> GDVVEAIEGAVARVADTISSGPTNSQAVPALTAVETGHTSQVVPGDTMQTRHVKNYHSRSESTIENFLSRSACVYMGEYYTTNTDETKRFASWTINARRMVQMRRKLEMFTYVRFDVEVTFVITSKQDQGTQLGQDMPPLTHQIMYIPPGGPIPKSTTDYAWQTSTNPSIFWTEGNAPPRMSIPFVSIGNAYSNFYDGWSHFSQNGVYGYNTLNNMGQLYMRHVNGPSPLPMTSIVRVYFKPKHVKAWVPRPPRLCQYKNASTVNFSSTNITDKRDSITHVPDTVKPDVTTH;> SPSAEECGYSDRVRSITLGNSTITTQECANVVVAYGRWPEYLSDKEATAEDQPTQPDVATCRFYTLESVTWEKDSPGWWWKFPDALKDMGLFGQNMYYHYLGRAGYTIHVQCNASKFHQGCLLVVCVPEAEMGCSDVGGTVNEHAISEGEIAKKFSATATNGAHTVQSIVTNAGMGVGVGNLTIYPHQWVNLRTNNSATIVMPYINSVPMDNMFRHHNFTLMIIPFVSLDYSSDASTYVPITVTVAPMCAEYNGLRLATSLQ;> GLPVMNTPGSNQFLTSDDFQSPSAMPQFDVTPELDIPGEVKNLMEIAEVDSVVPVNNVVGKLDTMDIFRIPVQSGNHQSTQVFGFQVQPGLDSVFKHTLLGEILNYYAHWSGSVKLTFVFCGSAMATGKFLLAYSPPGANAPKTRKDAMLGTHVIWDVGLQSSCVLCIPWISQTHYRLVHQDEYTSAGNVTCWYQTGIVVPAGTPTLCSIMCFVSACNDFSVRLLKDTPFIEQSALLQ;> MGAQVSTQKTGAHETGLNASGNSIIHYTNINYYKDAASNSANRQDFTQDPGKFTEPVKDIMIKSMPALN;> MGCVAETGDCGLPPDVPNAQPALEGRTSFPEDTVITYKCEESFVKIPGEKDSVICLKGSQWSDIEEFCNRSCEVPTRLNSASLKQPYITQNYFPVGTVVEYECRPGYRREPSLSPKLTCLQNLKWSTAVEFCKKKSCPNPGEIRNGQIDVPGGILFGATISFSCNTGYKLFGSTSSFCLISGSSVQWSDPLPECREIYCPAPPQIDNGIIQGERDHYGYRQSVTYACNKGFTMIGEHSIYCTVNNDEGEWSGPPPECRGGTKHHHHHH

Echoviruses, for which there are currently no approved vaccines or drugs, are responsible for a range of human diseases, for example echovirus 11 (E11) is a major cause of serious neonatal morbidity and mortality. Decay-accelerating factor (DAF, also known as CD55) is an attachment receptor for E11. The capsid consists of 60 identical protomers arranged with icosahedral symmetry and each protomer is composed of four capsid proteins, VP1–4, derived from the P1 polyprotein. DAF is one of the regulators of the complement system, inhibiting formation of the complement convertases in both the classical and alternative pathways.

The cryo-EM structure of the E11-DAF complex at neutral pH (pH 7.4) was determined at a nominal gold-standard resolution of 3.1 Å. In contrast the density for the DAF was weak. Whilst at low resolution the molecular envelope was clear, at high resolution the density became fragmentary at a contour level where the capsid density was still continuous. It was clear that this was in substantial part because the DAF bound close to the icosahedral 2-fold axes, so that at most only 30 DAFs could be bound per particle, in particular, SCR domains 2 and 3 of the 2-fold related DAF molecules clash. As expected for engagement with an attachment receptor with relatively weak binding (reported KD for E11 ∼3.0 μm), which is not responsible for internalisation and genome release, the E11 structure is in its un-expanded state with the natural pocket factor (modelled as sphingosine) bound in the VP1 pocket. DAF binds E11 at the southern rim of the canyon, rather than into the canyon itself. The footprint of the DAF receptor on the virus is ~900 Å2. The VP2 EF loop of E11 and SCR 3 of DAF dominate the interaction, although the VP3 BC loop of E11 and DAF SCR 4 are also involved. As a result of the differences a maximum of 30 DAF molecules can attach to E11, due to steric clashes near the 2-fold axis, whereas 60 copies of DAF can attach to the capsid in the E6 pose.The two main enzymes responsible for PI(3,4,5)P3 degradation are the tumor suppressor phosphatase and tensin homolog (PTEN), which removes the 3-phosphate (3 P) and the SH2-containing inositol 5-phosphatase (SHIP), which dephosphorylates the 5 P to generate PI(3,4)P2. The SHIP Ptase domain belongs to a family of Mg2+-dependent inositol phosphatases with specificity for 5 P dephosphorylation of inositol rings. Here, we report the crystal structure of SHIP2 containing the 5-Ptase and a C2 domain (Ptase-C2), revealing that the two domains tightly associate via an extensive interface. Importantly, even in the absence of a localization effect, the C2 domain provides activating signals to the Ptase active site, resulting in a significant increase in catalytic turnover.

Co-crystallization experiments using the catalytically inactive SHIP Ptase-C2 D607A mutant with Mg2+ and substrate failed to reveal clear electron density for the substrate. Although our co-crystallization experiments did not reveal bound substrate they did exhibit electron density corresponding to a Mg2+ ion and a phosphate group. The Mg2+ ion is on average displaced by 1.3 Å and the phosphate by 1.7 Å compared to the Mg2+ and 5 P positions in our model. The position of the phosphate does not leave space for an attacking water bound to D607, hence this could represent the post-catalysis positions of the Mg2+ and 5 P. Similar to a recent structure of INPP5B, we observe in our Ptase-C2 D607A structure the Mg2+ displaced on average by 1.3 Å from the A towards the B-site and a phosphate group shifted by 1.7 Å from the 5 P location towards the attacking water. As suggested by Mills et al. (2016) this likely represents the post-cleavage position for Mg2+ and the 5 P, since there is no longer space for the attacking water. We note that the movement of the Mg2+ seen in INPP5B and SHIP2 from the A towards the B-site is opposite to the B to A-site movement proposed to occur during catalysis in AP nucleases. In this complex the catalytic base D607 stabilizes a water molecule for 5 P attack.

>[8x]GPEPDMISVFIGTWNMGSVPPPKNVTSWFTSKGLGKTLDEVTVTIPHDIYVFGTQENSVGDREWLDLLRGGLKELTDLDYRPIAMQSLWNIKVAVLVKPEHENRISHVSTSSVKTGIANTLGNKGAVGVSFMFNGTSFGFVNCHLTSGNEKTARRNQNYLDILRLLSLGDRQLNAFDISLRFTHLFWFGALNYRLDMDIQEILNYISRKEFEPLLRVDQLNLEREKHKVFLRFSEEEISFPPTYRYERGSRDTYAWHKQKPTGVRTNVPSWCDRILWKSYPETHIICNSYGCTDDIVTSDHSPVFGTFEVGVTSQFISKKGLSKTSDQAYIEFESIEAIVKTASRTKFFIEFYSTCLEEYKKSFENDAQSSDNINFLKVQWSSRQLPTLKPILADIEYLQDQHLLLTVKSMDGYESYGECVVALKSMIGSTAQQFLTFLSHRGEETGNIRGSMKVRVPTER> ASRSQAEDVRVEGSFPVTMLPGDGVGPELMHAVKEVFKAAAVPVEFQEHHLSEVQNMASEEKLEQVLSSMKENKVAIIGKIHTPMEYKGELASYDMRLRRKLDLFANVVHVKSLPGYMTRHNNLDLVIIREQTEGEYSSLEHESARGVIECLKIVTRAKSQRIAKFAFDYA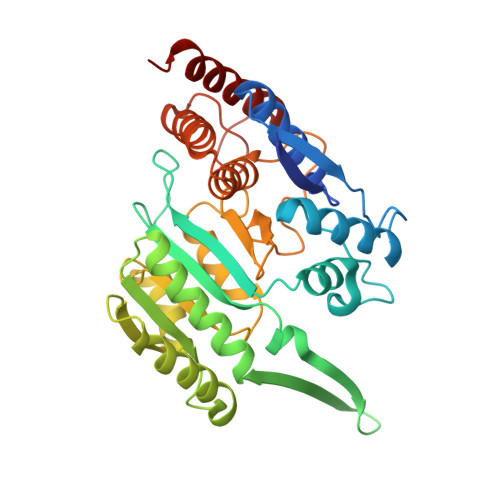TKKGRGKVTAVHKANIMKLGDGLFLQCCEEVAELYPKIKFETMIIDNCCMQLVQNPYQFDVLVMPNLYGNIIDNLAAGLVGGAGVVPGESYSAEYAVFETGARHPFAQAVGRNIANPTAMLLSASNMLRHLNLEYHSSMIADAVKKVIKVGKVRTSDMGGYATCHDFTEEICRRVKDLDENLYFQ>[2x]MLGGVRDVLGTLSAVWESGGTAGVGTVVRTFRSAPRPAGASMVVAPDGTVSGSVSGGCVEGAVYDLATEVVATGTPVLQRYGVSDDDAFEVGLTCGGILDVFVEPVSQKTFPQLGAIRDDIEAQRPVAVATVITHPDAQWIGRRLVVHTDEVAGSLGSSRADAAVTDDA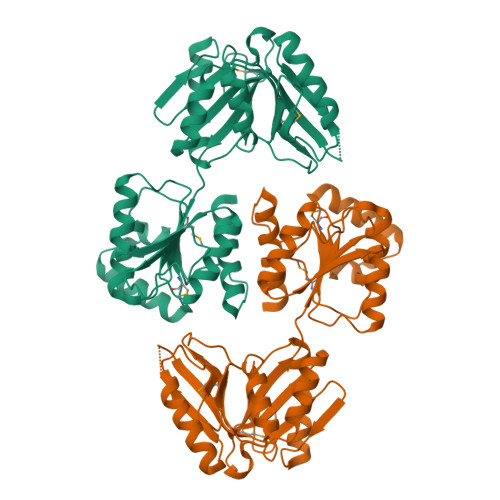RGLLAAGRSEVLTYGPDGQRRGEGMEVFVSSYAPRPRMLVFGAIDFAAAVAQQGAFLGYRVTVCDARPVFATTARFPTADEVVVDWPHRYLAAQAEAGAIDARTVVCVLTHDPKFDVPLLEVALRLPDIAYIGAMGSRRTHEDRLARLREAGLTEEELARLSSPIGLDLGGRTPEETAVSIAAEIIAKRWGGEGRPLAETGGRIHHELGEHESAPAS>MFENITAAPADPILGLADLFRADERPGKINLGIGVYKDETGKTPVLTSVKKAEQYLLENETTKNYLGIDGIPEFGRCTQELLFGKGSALINDKRARTAQTPGGTGALRVAADFLAKNTSVKRVWVSNASWPNHKSVFNSAGLEVREYAYYDAENHTLDFDALINSLNEAQAGDVVLFHGCCHNATGIDPTLEQWQTLAQLSVEKGWLPLF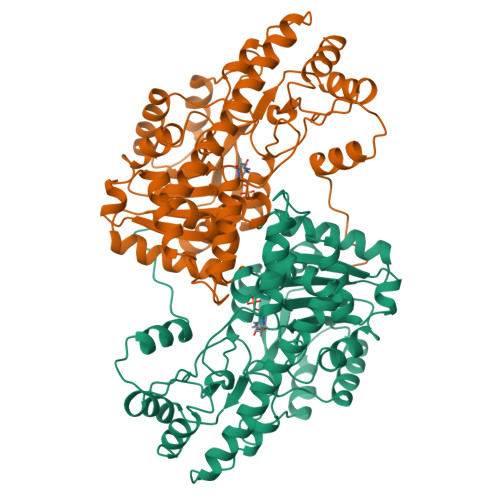DFAYQGFARGLEEDAEGLRAFAAMHKELIVASSYSKNFGLYNERVGACTLVAADSETVDRAFSQMKAAIRANYSNPPAHGASVVATILSNDALRAIWEQELTDMRQRIQRMRQLFVNTLQEKGANRDFSFIIKQNGMFSFSGLTKEQVLRLREEFGVYAVASGRVNVAGMTPDNMAPLCEAIVAVL[2x]>[2x]MHHHHHHSSGLVPRGSHMISKEYHIDEEVGFALPNPQENLPDFYNDWMFIAKHLPDLIESGQLRERVEKLNMLSIDHLTDHKSQRLARLVLGCITMAYVWGKGHGDVRKVLPRNIAVPYCQLSKKLELPPILVYADCVLANWKKKDPNKPLTYENMDVLFSFRDGDCSKGFFLVSLLVEIAAASAIKVIPTVFKAMQMQERDTLLKALLEIASCLEKALQVFH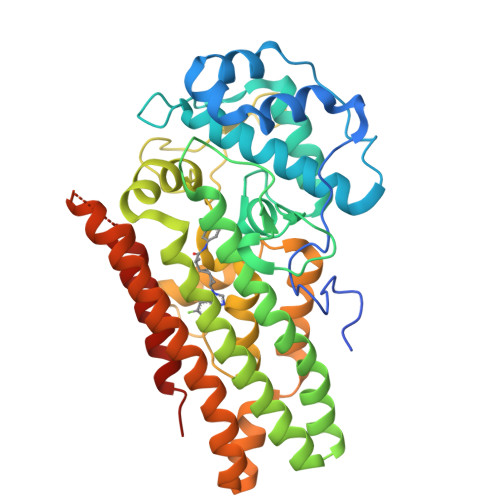QIHDHVNPKAFFSVLRIYLSGWKGNPQLSDGLVYEGFWEDPKEFAGGSAGQSSVFQCFDVLLGIQQTAGGGHAAQFLQDMRRYMPPAHRNFLCSLESNPSVREFVLSKGDAGLREAYDACVKALVSLRSYHLQIVTKYILIPASQQPKENKTSEDPSKLEAKGTGGTDLMNFLKTVRSTTEKSLLKEG>MEDGTPKHIIQMTGFKMEEKEALVKLLLKLDCTFIKSEKYKNCTHLIAERLCKSEKFLAACAAGKWILTKDYIIHSAKSGRWLDETTYEWGYKIEKDSRYSPQMQSAPKRWREELKRTGAPGAFHRWKVVLLVRTDKRSDSLIRVLEAGKANVILPKSSPSGITHVIASNARIKAEKEKDNFKAPFYPIQYLGDFLLEKLEHHHHHH[2x];>[2x]SDSCNSSSSDIIRDLLE

Rad18 interacts with the SMC5/6 localization factor 1 (SLF1) to recruit the SMC5/6 complex to DNA damage sites for repair. Previous studies have shown that the tandem BRCA1 C-Terminal (BRCT) domain repeat (tBRCT) at the SLF1 N-terminus (SLF1tBRCT) plays a critical role in the Rad18-SLF1 association. Our structure and biochemical studies demonstrate that SLF1tBRCT interacts with two phosphoserines and adjacent residues in Rad18 for high-affinity and specificity Rad18 recognition. We found that SLF1tBRCT utilizes mechanisms common among tBRCTs as well as unique ones for Rad18 binding, the latter include interactions with an α-helical structure in Rad18 that has not been observed in other tBRCT-bound ligand proteins.

To further clarify the roles of Ser442 and 444 phosphorylation in the Rad18-SLF1 interaction, we co-crystallized SLF1tBRCT with the singularly phosphorylated Rad18-pS442 peptide and determined its structure to a resolution of 1.62 Å. Two SLF1tBRCT molecules were found in the asymmetric unit and electron densities for the Rad18-pSer442 peptide were found on both of them. The structure and crystal packing of the SLF1tBRCT-Rad18-pS442 complex are very similar to the SLF1tBRCT-Rad18-2P complex. Compared to the SLF1tBRCT-Rad18-2P complex, little structural differences were observed even for the SLF1 Arg50 and Rad18 Arg448 side chains, which interact with the pS444 phosphate group in the Rad18-2P peptide. The electron densities for the Rad18-pS442 peptide are weaker compared to electron densities for the Rad18-2P peptide, especially at the N-terminal region where Ser442 and Ser444 reside. Such a difference in density is in line with the reduced affinity of the Rad18-pS442 peptide toward SLF1tBRCT and supports the function of Ser444 phosphorylation in enhancing the Rad18-SLF1tBRCT binding. Electron densities for the Arg448 side chain in the Rad18-pS442 peptide are also weaker, consistent with the lack of Arg448-pS444 interaction in this peptide. The N-terminus of the helix and neighboring region pack against the SLF1 52-55 region, with the pS444 carbonyl and Asp445 amide groups in this region forming hydrogen bonds with the mainchain amide and carbonyl groups of Lys53 in SLF1, respectively. The same regions in the Rad18-pS442 peptide form virtually identical interactions with SLF1tBRCT, although the pS444-Arg448 interaction is absent in this peptide. Our binding experiments suggest that Ser442 phosphorylation is critical and sufficient for strong Rad18-SLF1tBRCT association.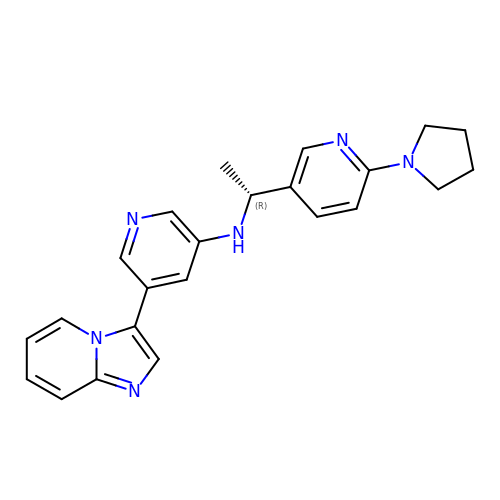5-imidazo[1,2-a]pyridin-3-yl-~{N}-[(1~{R})-1-(6-pyrrolidin-1-ylpyridin-3-yl)ethyl]pyridin-3-amine | C23 H24 N6 | XVRRLWMWIRHFPC-QGZVFWFLSA-N>DEMAHRRYCKRTIPPGYKVDQVFGPRTKGKEGNFGDDKMNEEGIKDGRVTAMLNLVPSSHACLFGSRVTPKLQPDGLHLKFEFT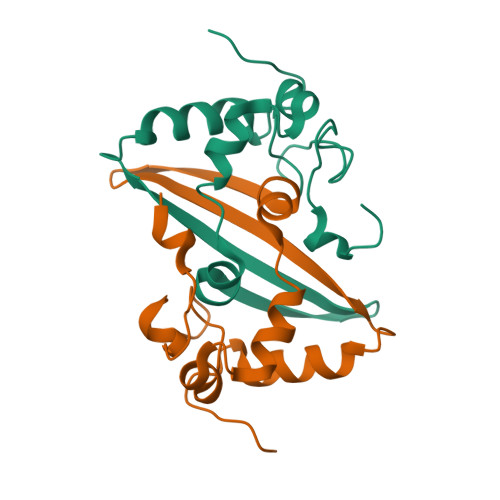TVVPRDDPQFDNYVKICDQCVDGVGTRPKD[8x]>AHHHHHHPCCSNPCQNRGECMSTGFDQYKCDCTRTGFYGENCTTPEFLTRIKLLLKPTPNTVHYILTHFKGVWNIVNNIPFLRSLIMKYVLTSRSYLIDSPPTYNVHYGYKSWEAFSNLSYYTRALPPVADDCPTPMGVKGNKELPDSKEVLEKVLLRREFIPDPQGSNMMFAFFAQHFTHQFFKTDHKRGPGFTRGLGHGVDLNHIYGETLDRQHKLRLFKDGKLKYQVIGGEVYPPTVKDTQVEMIYPPHIPENLQFAVGQEVFGLVPGLMMYATIWLREHNRVCDILKQEHPEWGDEQLFQTSRLILIGETIKIVIEDYVQHLSGYHFKLKFDPELLFNQQFQYQNRIASEFNTLYHWHPLLPDTFNIEDQEYSFKQFLYNNSILLEHGLTQFVESFTRQIAGRVAGGRNVPIAVQAVAKASIDQSREMKYQSLNEYRKRFSLKPYTSFEELTGEKEMAAELKALYSDIDVMELYPALLVEKPHPDAIFGETMVELGAPFSLKGLMGNPICSPQYWKPSTFGGEVGFKIINTASIQSLICNN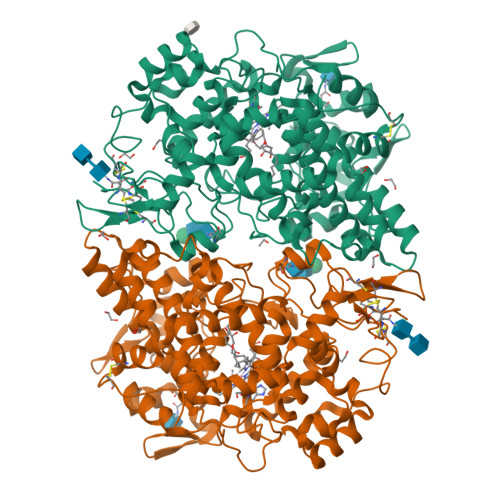VKGCPFTSFNVQDPQPTKTATINASASHSRLDDINPTVLIKRRSTEL[2x]> MSDTMVVNGSGGVPAFLFSGSTLSSYRPNFEANSITIALPHYVNLPGRSNFKLMYIMGFPIDTEMEKDSEYSNKIRQESKISKTEGTVCYEQKITVETGQEKDGVKVYRVMVLEGTIAESIEHLDKKENEDILNNNRNRIVLADNTVINFDNISQLKEFLRRSVNIVDHDIFSSNGFEGFNPTSHFPSNPSSDYFNSTGVTFGSGVDLGQRSKQDLLNDGVPQYIADRLDGYYMLRGKEAYDKVRTAPLTLSDNEAHLLSNIYIDKFSHKIEGLFNDANIGLRFCDLPLRTRTALVSIGYQKGFKLSRTA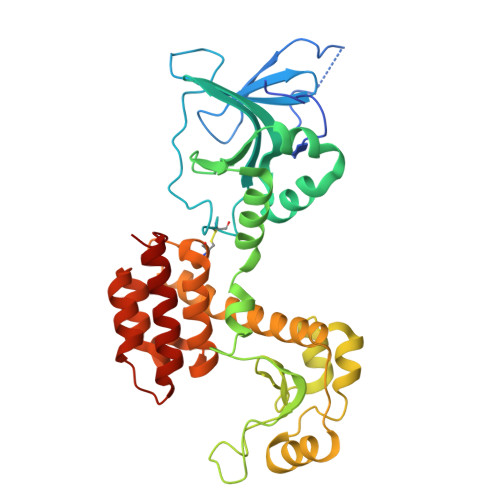PTVWNKVIAKDWNGLVNAFNNIVDGMSDRRKREGALVQKDIDSGLLK> GPSQPKVPEWVNTPSTCCLKYYEKVLPRRLVVGYRKALNCHLPAIIFVTKRNREVCTN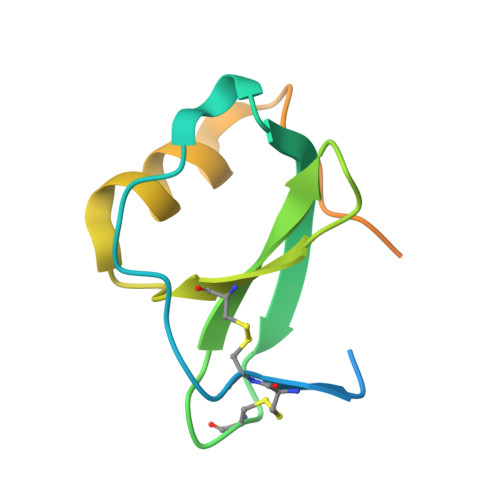PNDDWVQEYIKDPNLPLLPTRNLSTVKIITAKNGQPQLLNSQ> MVRIDVISIFPAYLDPIRQSL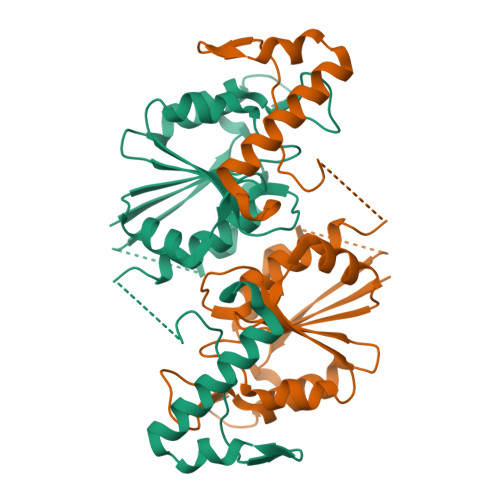PGKAIDAGIVSVEVHDLRNWTHDVHRSVDDSPYGGGPGMVMKAPVWGEALDEICSEETLLVVPTPAGRLFDQRTAQRWSTERHLVFACGRYEGIDQRVVDDAARRMRVEEVSIGDYVLNGGEAATLVMVEAVVRLLPDVLGNPASHQQDSHSDGLLEGPSYTRPPSWRGLDVPPVLLSGDHAKVAAWRHEQALQRTRERRPDLLDAGHHHHHH> MVPISPIETVPVKLKPGMDGPKVKQWPLTEEKIKALVEICTEMEKEGKISKIGPENPYNTPVFAIKKKDSTKWRKLVDFRELNKRTQDFWEVQLGIPHPAGLKKKKSVTVLDVGDAYFSVPLDEDFRKYTAFTIPSINNETPGIRYQY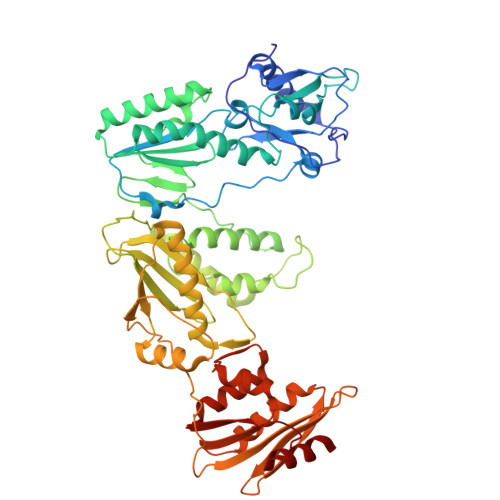NVLPQGWKGSPAIFQSSMTKILEPFKKQNPDIVIYQYMDDLYVGSDLEIGQHRTKIEELRQHLLRWGLTTPDKKHQKEPPFLWMGYELHPDKWTVQPIVLPEKDSWTVNDICKLVGKLNWASQIYPGIKVRQLSKLLRGTKALTEVIPLTEEAELELAENREILKEPVHGVYYDPSKDLIAEIQKQGQGQWTYQIYQEPFKNLKTGKYARMRGAHTNDVKQLTEAVQKITTESIVIWGKTPKFKLPIQKETWETWWTEYWQATWIPEWEFVNTPPLVKLWYQLEKEPIVGAETFYVDGAANRETKLGKAGYVTNKGRQKVVPLTNTTNQKTELQAIYLALQDSGLEVNIVTNSQYALGIIQAQPDKSESELVNQIIEQLIKKEKVYLAWVPAHKGIGGNEQVDKLVSAG> MSMLKREDWYDLTRTTNWTPKYVTENELFPEEMSGARGISMEAWEKYDEPYKITYPEYVSIQREKDSGAYSIKAALERDGFVDRADPGWVSTMQLHFGAIALEEYAASTAEARMARFAKAPGNRNMATFGMMDENRHGQIQLYFPYANVKRSRKWDWAHKAIHTNEWAAIAARSFFDDMMMTRDSVAVSIMLTFAFETGFGNMQFLGLAADAAEAGDHTFASLISSIQTDESRHAQQGGPSLKILVENGKKDEAQQMVDVAIWRSWKLFSVLTGPIMDYYTPLESRNQSFKEFMLEWIVAQFERQLLDLGLDKPWYWDQFMQDLDETHHGMHLGVWYWRPTVWWDPAAGVSPEEREWLEEKYPGWNDTWGQCWDVITDNLVNGKPELTVPETLP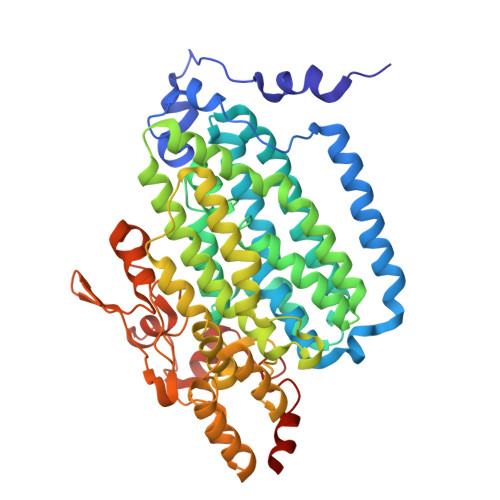TICNMCNLPIAHTPGNKWNVKDYQLEYEGRLYHFGSEADRWCFQIDPERYENHTNLVDRFLKGEIQPADLAGALMYMSLEPGVMGDDAHDYEWVKAYQKKTNAA S-layer proteins (SLPs) are self-assembling, crystalline proteins coating the cell surfaces of many prokaryotes. We determined the atomic resolution structures of all functional domains (I-III from N- to C-termini) present in the three S-layer proteins SlpA_ac, SlpX_ac, and SlpA_amy. The Lactobacillus S-layers are anchored to the cell wall through interaction with teichoic acids (TA), either lipoteichoic acid (LTA) or wall teichoic acid (WTA).

The full-length SlpX_ac shows differences in structure and domain arrangement compared to the SlpA architecture. SlpX_ac_I accommodates a similar fold to both SlpA_II, with SlpX_ac_I being slightly larger. Likewise, SlpX_ac_I is structurally conserved (RMSD: 2.6 Å) to SlpA_ac_II, indicating the possible dimer formation as observed for SlpA_ac_I. Therefore, the SlpX homodimer might be incorporated within the assembled SlpA layer via the two described interfaces.

>MGDTAVNVGSAAGTGANTTNTTTQAPQNKPYFTYNNEIIGEATQSNPLGNVVRTTISFKSDDKVSDLISTISKAVQFHKNNSASGENVTINENDFINQLKANGVTVKTVQPSNKNEKAYEAIDKVPSTSFNITLSATGDNNQTATIQIPMVPQGLEHHHHHH[2x]> GPEKYKNILEKLEWYKNKSSEKYEFGIYEIDKREVFITTKYSYGFVNNKPLLPGHILLTTLKKKKHYNDLDIEEIIDINLLCNFMCYIMGNLFNTTDFSIAIQDGKEAGQTVDHVHIHIIPRKINDYKNNDNIYNDMNKINLGYGKNIICNSCNNTINVCSQNEIERNFKLEEFNTSIRSIEQMEEEANL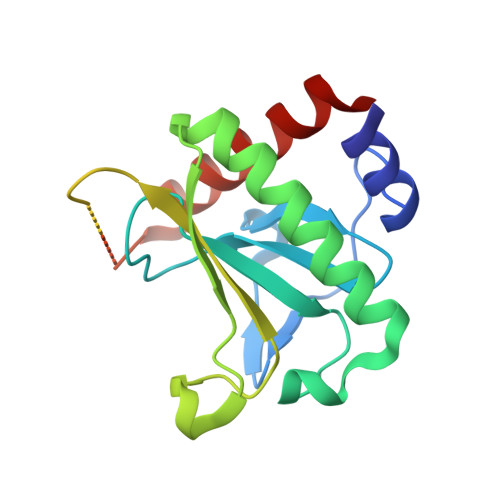IKSYINEKFSS5'-([(3S)-3-amino-3-carboxypropyl]{3-[(4R)-7,8-dichloro-1,2,3,4-tetrahydroisoquinolin-4-yl]propyl}amino)-5'-deoxyadenosine | C26 H34 Cl2 N8 O5 | 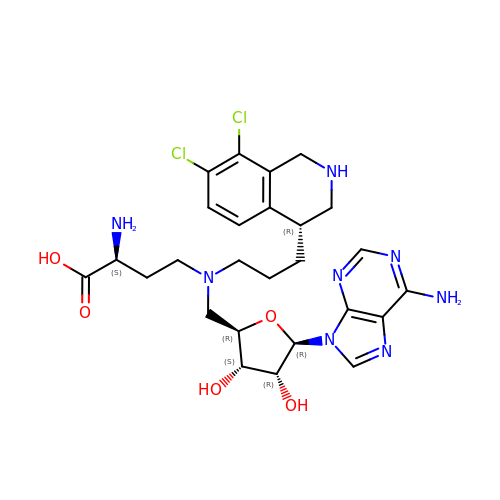LJUSEDZPCVZRMF-RYHYOYCJSA-N>GSTPAAPLDVKCLEANKDYIIISWKQPAVDGGSPILGYFIDKCEVGTDSWSQCNDTPVKFARFPVTGLIEGRSYIFRVRAVNKMGIGFPSRVSEPVAALDPAEKA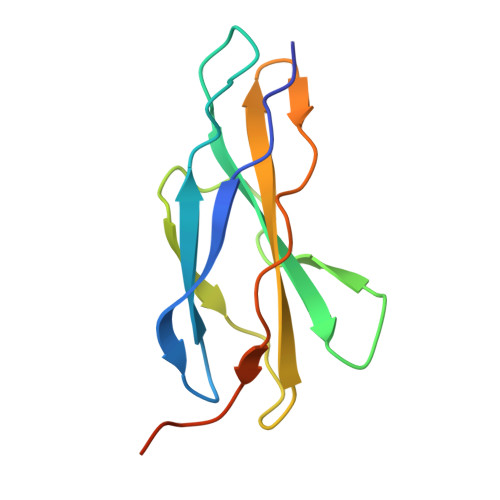RLKSRPS[4x]> ESMITSIGNPVQVLKVTETFGTWIRESANKSDDRIWVTEHFSGIMVKEFKDQPSLLNGSYTFIHLPYYFHGCGHVVYNNSLYYHKGGSNTLVRFEFGQETSQTLKLENALYFDRKYLFANSKTYFNLAVDEKGLWIIYASSVDGSSILVAQLDERTFS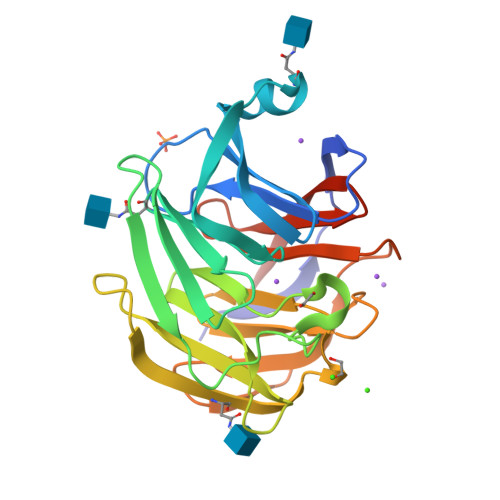VVQHVNTTYPKSKAGNAFIARGILYVTDTKDMRVTFAFDLLGGKQINANFDLRTSQSVLAMLAYNMRDQHLYSWEDGHLMLYPVQFLSTTLNQ>[2x]MTGPHAAGGSNHRTARLVAIIAGLLGTLMAIATPLLPVEQTTAELNWPQNGVWQSVDAPLIGYVATDLTVTVPCQAAAGLVGPENRNRSVLLSTVPKQAPKAIDRGLLIERINNDLTVIVRNTPVVSAPLEQVLSPDCRYLTFTAHADKVTGEFVGLTQGPDDDDPGEAVRGERSGYDFRPQIVGVFTDLSGPAPEGLQLSATIDTRYSTSPTLLKLLAMIVGVAMTVIALGALHVLDCADGRRHKRFLPSRWWSMTPLDGLVSAMLVWWHFVGANTADDGYILTMARVSEHAGYMANYYRWFGTPESPFGWYYDLLALWAHVSTASVWMRFPTLLMGLACWWVISREVIPRLGAAAKHSRAAAWTAAGLFLAFWLPLNNGLRPEPIIALGILLTWCSVERGVATSRLLPVAVAIIIGALTLFSGPTGIAAVGALLVAIGPLKTIVAAHVSRFGYWALLAPIAAAGTVTIFLIFRDQTLAAELQASSFKSAVGPSLAWFDEHIRYSRLFTTSPDGSVARRFAVLTLLLALAVSIAMTLRKGRIPGTALGPSRRIIGITIISFLAMMFTPTKWTHHFGVFAGLAGCLGALAAVAVTTTAMKSRRNRTVFGAAVLFVTALSFATVNGWWYVSNFGVPWSN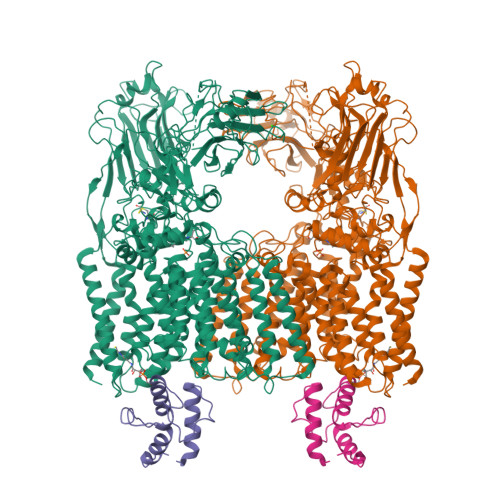SFPEFKFGFTTMLLGLSVLALLVAAWFHFSGRDVSPDRPQRRWQRLLVAPLAVATWALVIFEVVSLTLGMINQYPAWSVGRSNLNALTGKTCGLANDVLVEQNANAGMLTPIGEPAGQALGAVTSLGFGPNGIPSDVSADPVMEQPGTDNFADSDSGVVTGTEVGTEGGTTAAAGINGSRARLPYGLNPATTPVLGSWRSGTQQPAVLRSAWYRLPDRDQAGPLLVVSAAGRFDQGEVEVQWATDEQAAANEPGGSITFGDVGAAPAWRNLRAPLSSIPPEATQIRLVASDDDLAPQHWIALTPPRIPELRTLQEVVGSSDPVMLDWLVGLAFPCQRPFDHRYGVVEVPKWRILPDRFGAEANSPVMDYLGGGPLGITELLLRPSSVPTYLKDDWYRDWGSLQRLTPWYPDAQPARLDLGTATRSGWWSPAPLRLSHHHHHHHHHH;>[2x]MAATQEEIIAGLAEIIEEVTGIEPSEVTPEKSFVDDLDIDSLSMVEIAVQTEDKYGVKIPDEDLAGLRTVGDVVAYIQKLEEENPEAAAALREKFAADQ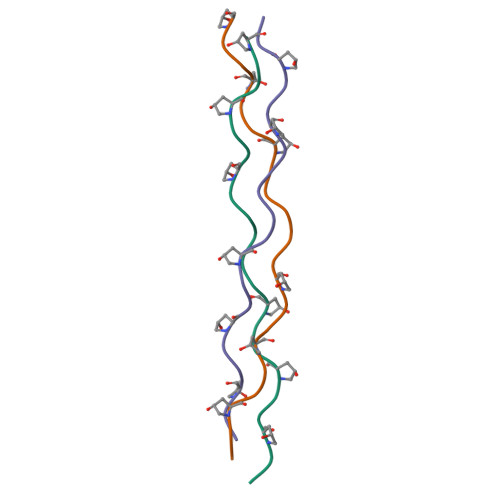>[3x]XGPPGPPGFPGERGPPGPPGPPX> AEGDDPAKAAFNSLQASATEYIGYAWAMVVVIVGATIGIKLFKKFTS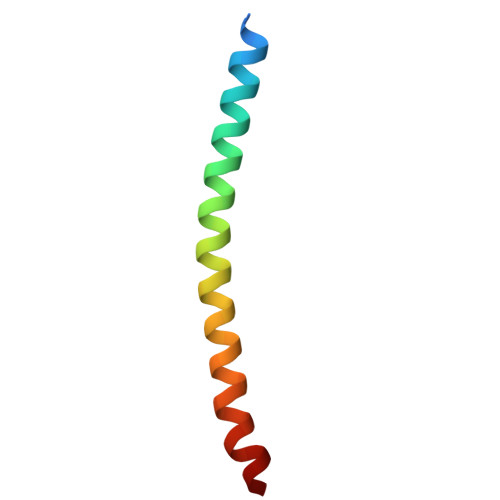KAS> MDENAKEPENRFLRKLLKPDIERERLKAVNSIISIVFGTRRIAWAHLDRKLTVLDWQQSDRWSLMRGIYSSS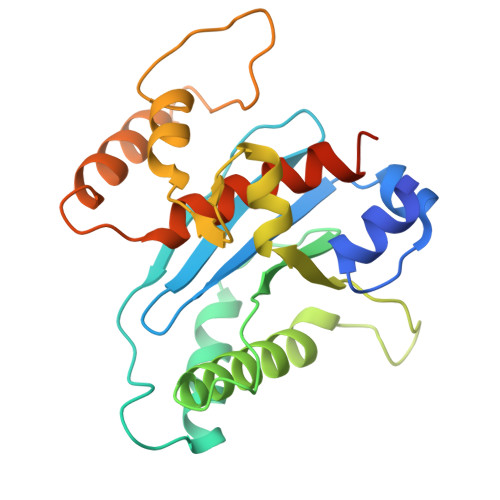VYLEEISSIISKMPKADFYVLEKTGLSIQNSSLFPILLHFHIMEAMLYALLNKTFAQDGQHQVLSMNRNAVGKHFELMIGDSRTSGKELVKQFLFDSILKADPRVFFPSDKIVHYRQMFLSTELQRVEELYDSLLQAIAFYELAVFDSQPLEHHHHHHHH>MSYMLPHLHNGWQVDQAILSEEDRVVVIRFGHDWDPTCMKMDEVLYSIAEKVKNFAVIYLVDITEVPDFNKMYELYDPCTVMFFFRNKHIMIDLGTGNNNKINWAMEDKQEMVDIIETVYRGARKGRGLVVSPKDYSTKYRY[3x];>[3x]AEEEL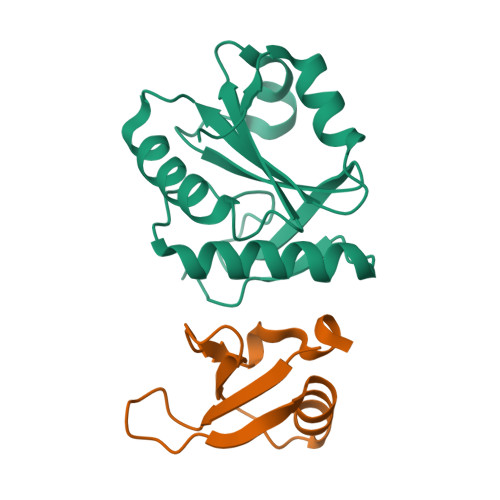ETPTPTQRGEAESRGDGLVDVMWEYKWENTGDAELYGPFTSAQMQTWVSEGYFPDGVYCRKLDPPGGQFYNSKRIDFDLYT> GSVGPKTGEENQVLVPNLNPTPENLEVVGDGFKITSSINLVGEEEADENAVNALREFLTANNIEINSENDPNSTTLIIGEVDDDIPELDEALNGTTAENLKEEGYALVSNDGKIAIEGKDGDGTFYGVQTFKQLVKESNIPEVNITDYPTVSARGIVEGFYGTPWTHQDRLDQIKFYGENKLNTYIYAPKDDPYHREKWREPYPESEMQRMQELINASAENKVDFVFGISPGIDIRFDGDAGEEDFNHLITKAESLYDMGVRSFAIYWDNIQDKSAAKHAQVLNRFNEEFVKAKGDVKPLITVPTEYDTGAMVSNGQPRAYTRIFAETVDPSIEVMWTGPGVVTNEIPLSDAQLISGIYDRNMAVWWNYPVTDYFKGKLALGPMHGLDKGLNQYVDFFTVNPMEHAELSKISIHTAADYSWNMDNYDYDKAWNRAIDMLYGDLAEDMKVFANHSTRMDNKTWAKSGREDAPELRAKMDELWNKLSSKEDASALIEELYGEFARMEEACNNLKANLPEVALEECSRQLDELITLAQGDKASLDMIVAQLNEDTEAYESAKEIAQNKLNTALSSFAVISEKVAQSFIQEALS;> VPYSSAQ

Reversible protein O-GlcNAcylation is achieved by the action of two enzymes, O-GlcNAc transferase (OGT) and O-GlcNAcase (OGA). Although it is unclear whether CpOGA is a physiological OGA, it shows significant in vitro O-GlcNAcase activity on O-GlcNAc proteins in lysates from human cell lines and possesses a putative substrate-binding groove conserved with hOGA (Rao et al., 2006; Schimpl et al., 2010). We report the molecular details of the interaction of a bacterial O-GlcNAcase homolog with three different synthetic glycopeptides derived from characterized O-GlcNAc sites in the human proteome. In addition to extensive contacts with the sugar, O-GlcNAcase recognizes the peptide backbone through hydrophobic interactions and intramolecular hydrogen bonds, while avoiding interactions with the glycopeptide side chains.

Here we report that CpOGA, like hOGA (Schimpl et al., 2010), possesses activity toward synthetic glycopeptides derived from validated O-GlcNAc sites in the human proteome, namely p53 (Ser149 [Yang et al., 2006]), TAK1-binding protein 1 (TAB1, Ser395 [Schimpl et al., 2010]), and hOGA itself (Ser405 [Lazarus et al., 2006]). To investigate the molecular basis of this substrate specificity, we exploited the catalytic acid mutant of CpOGA, D298N, which is inactive yet unaffected in its ability to bind substrate (Rao et al., 2006). We generated an alternative CpOGA crystal form with a highly accessible active site and determined the structures of CpOGA D298N in complex with the p53-, TAB1-, and hOGA-derived O-GlcNAc peptides. The O-GlcNAc sugar occupies the same position in all three structures (maximum atomic shift of 0.2 Å). Strikingly, the backbones of all three glycopeptides run in the same direction, together defining the −4 through +3 subsites, and adopt similar conformations near the O-GlcNAc site (maximum Cα shift of 1.8 Å for the −2 to +1 subsites). All three glycopeptides adopt a “V-shaped” conformation that allows the sugar to penetrate the OGA active site. Interestingly, for two of the peptides, this conformation appears to be stabilized by intramolecular hydrogen bonds. For the p53-derived glycopeptide, a hydrogen bond is observed between the aspartic acid in the −1 subsite and the threonine in the +1 subsite. Such intramolecular interactions may stabilize the OGA-bound conformation of these glycopeptides, explaining the significantly lower Kms compared to the TAB1-derived peptide. We tested this hypothesis by designing glycopeptide sequences that either disrupted (in case of the p53-derived peptide) or introduced (in case of the TAB1-derived peptide) such intramolecular interactions. Indeed, introducing a hydrogen bond acceptor in the TAB1 peptide leads to a 5-fold decrease in Km for hOGA, whereas disrupting the hydrogen bond in the p53-derived peptide, either by removing the hydrogen bond donor or acceptor, leads to an 85-fold increase in Km.> MANVPWAEVCEKFQAALALSRVELHKNPEKEPYKSKYSARALLEEVKALLGPAPEDEDERPEAEDGPGAGDHALGLPAEVVEPEGPVAQRAVRLAVIEFHLGVNHIDTEELSAGEEHLVKCLRLLRRYRLSHDCISLCIQAQNNLGILWSEREEIETAQAYLESSEALYNQYMKEVGSPPLDPTERFLPEEEKLTEQERSKRFEKVYTHNLYYLAQVYQHLEMFEKAAHYCHSTLKRQLEHNAYHPIEWAINAATLSQFYINKLCFMEARHCLSAANVIFGQTGKISATEDTPEAEGEVPELYHQRKGEIARCWIKYCLTLMQNAQLSMQDNIGELDLDKQSELRALRKKELDEEESIRKKAVQFGTGELCDAISAVEEKVSYLRPLDFEEARELFLLGQHYVFEAKEFFQIDGYVTDHIEVVQDHSALFKVLAFFETDMERRCKMHKRRIAMLEPLTVDLNPQYYLLVNRQIQFEIAHAYYDMMDLKVAIADRLRDPDSHIV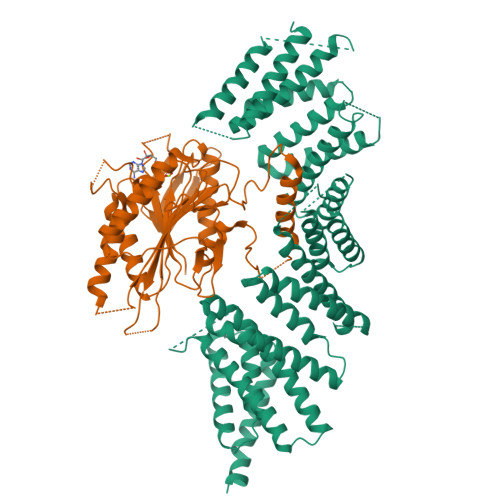KKINNLNKSALKYYQLFLDSLRDPNKVFPEHIGEDVLRPAMLAKFRVARLYGKIITADPKKELENLATSLEHYKFIVDYCEKHPEAAQEIEVELELSKEMVSLLPTKMERFRTKMALT;> MAPGSKTELRSVTNGQSNQPSNEGDAIKVFVRIRPPAERSGSADGEQNLSLSVLSSTSLRLHSNPEPKTFTFDHVADVDTTQESVFATVAKSIVESCMSGYNGTIFAYGQTGSGKTFTMMGPSESDNFSHNLRGVIPRSFEYLFSLIDREKEKAGAGKSFLSKCSFIEIYNEQIYDLLDSASAGLYLREHIKKGVFVVGAVEQVVTSAAEAYQVLSGGWRNRRVASTSMNRESSRSHAVFTITIESMEKCNEIVNIRTSLLNLVDLAGSERQKDTHAEGMRLKEAGNINRSLSTLGQVITALVDVGNGKQRHVSYRDSKLTFLLRDSLGGNAKTAIIANVHPGSRSFGETLSTLNFAQRAKLIKNKAVVNEDTQCLEHHHHHH>[6x]LELDESAAQKFVKQVIREAFLQDASDIHIEPRQNDVQVRLRIDGALRPYSTLPKGALNAVISVVKIMGGLNIAEKRLPQDGRVRYREGAIDVDLRLSTLPTVYGEKAVMRLLKKASDIPEIEDLGFAPGVFERFKEVISKPYGIFLITGPTGSGKSFTTFSILKRIATPDKNTQT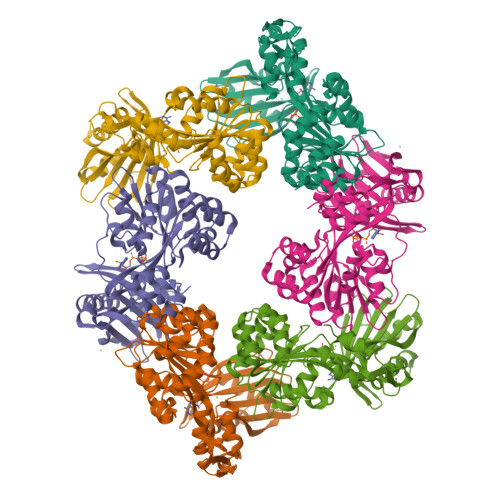IEDPVEYEIPGINQTQVNPQAGLTFARALRAFLRQDPDIIMVGEIRDSETAKIATEAALTGHLVIATLHTNDAAQAITRLDEMGVEPFNISAALIGVLSQRLVRRVCEHCKVEVKPDPETLRRLGLSEAEIQGARLYKGMGCERCGGTGYKGRYAIHELLVVDDEIRHAIVAGKSATEIKEIARRKGMKTLREDGLYKALQGITTLEEVLARTIE>MFIRIKCFSKQPIAKKVSREVSAYLEYTGNNTWEGHISGQGVSNLQTKLINVGKGVKVVCNYQDKVLFAIGNVAM[2x];>[4x]MQKQILTSQKRNMYILSRCKVLVKNGQVCHLHEDGNVYTVPYANTVFIGLAEGTSITNEAMSMLAANGVIVFWTKGGGYDMFAADIICHLPQADYRPTKYMQNWVRLWLDEEKKLSAAKEILKMRVDSLSTHVHDFGVDVENKRVSSIVNKFDKGVTQATSFESLLGHEGTFVKSLYKEYALEYEIEFKRDHKSADNYNKFLTLGNYYAYGIARSSLWALGIDNSFPLLHGSTRRGGLVFDVADIIKTSIILPLAFHAADQGMSNTEFKRSCV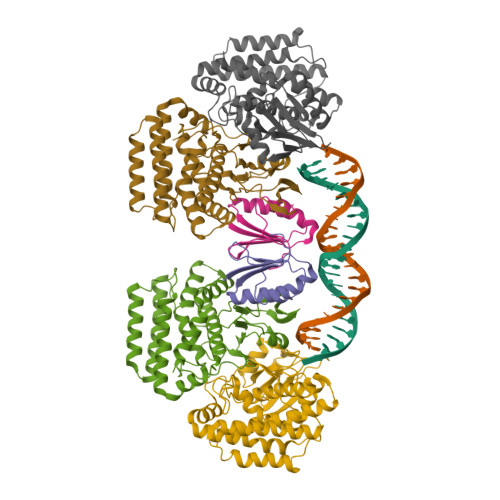AYFDKNDILAYLINNIKRLCME> VNGTLMQYFEWYTPNDGQHWKRLQNDAEHLSD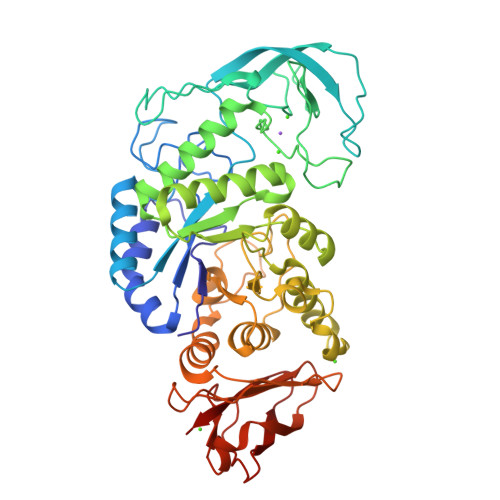IGITAVWIPPAYKGLSQSDNGYGPYDLYDLGEFQQKGTVRTKYGTKSELQDAIGSLHSRNVQVYGDVVLNHKAGADATEDVTAVEVNPANRNQETSEEYQIKAWTDFRFPGRGNTYSDFKWHWYHFDGADWDESRKISRIFKFRGEGKAWDWEVSSENGNYDYLMYADVDYDHPDVVAETKKWGIWYANELSLDGFRIDAAKHIKFSFLRDWVQAVRQATGKEMFTVAEYWQNNAGKLENYLNKTSFNQSVFDVPLHFNLQAASSQGGGYDMRKLLNGTVVSKHPLKSVTFVDNHDTQPGQSLESTVQTWFKPLAYAFILTRESGYPQVFYGDMYGTKGDSQREIPALKHKIEPILKARKQYAYGAQHDYFDHHDIVGWTREGDSSVANSGLAALITDGPGGAKRMYVGRQNAGETWHDITGNRSEPVVINSEGWGEFHVNGGSVSIYVQR> MAIITPALISALKTSFQKHFQDALATAPSTYLQVATVIPSTTASNTYGWLGQFPKLREWIGQRVIKDMAAQGYQITNKLFESTVGVKRTDIEDDNLGVYGPLMQEMGRAAGA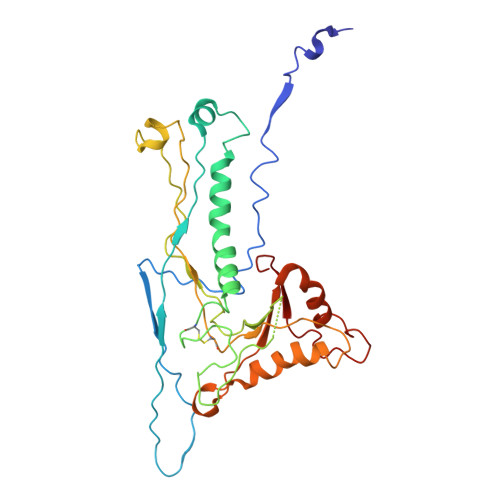HPDELVFALLKAGNANLCYDGQNFFDTDHPVYPNVDGTGTATTVSNLFAPAADPGAAWYLLDTSRSLKPLIYQERMKPSFTSMTKEDDEQVFMADEYRYGVRSRCNVGFGFWQLAAMSTEELNQVNFEKVYDAMRNQKADGGRPLDIRPNLLVVPTTLRSKAKEVVGVQRLANGADNPNFELVQVLDTAWLN4-[(6-ethenyl-7~{H}-purin-2-yl)amino]benzenesulfonamide | C13 H12 N6 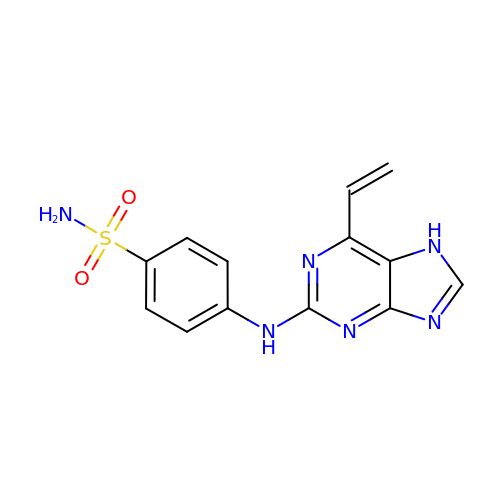O2 S | KGGMBTYAIOMGPI-UHFFFAOYSA-N>[4x]GAMGSMTDDKDVLRDVWFGRIPTCFTLYQDEITEREAEPYYLLLPRVSYLTLVTDKVKKHFQKVMRQEDISEIWFEYEGTPLKWHYPIGLLF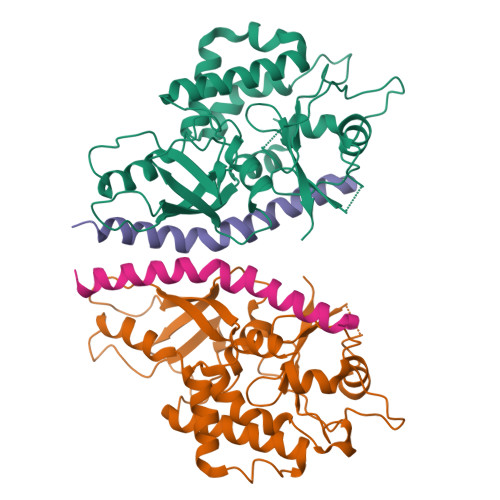DLLASSSALPWNITVHFKSFPEKDLLHCPSKDAIDAHFMSCMKEADALKHKSQVINEMQKKDHKQLWMGLQNDRFDQFWAINRKLMEYPAEENGFRYIPFRIYQTTTERPFIQKLFRPVAADGQLHTLGDLLKEVCPSAIDPEDGEKKNQVMIHGIEPMLETPLQWLSEHLSYPDNFLHISIIPQPTD;>GSMSSGLRAADFPRWKRHISEQLRRRDRLQRQAFEEIILQYNKLLEKSDLHSVLAQKLQAEKHDVPNRHEI[4x]R-2-PHENYL-PROPRIONIC ACID | 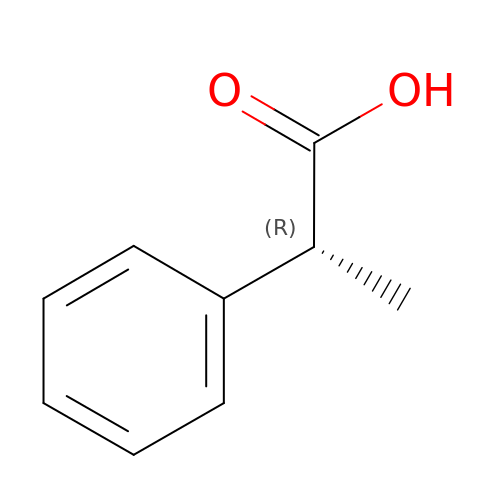C9 H10 O2 | YPGCWEMNNLXISK-SSDOTTSWSA-N> QDSTSDLIPAPPLSKVPLQQNFQDNQFQGKWYVVGLAGNAILREDKDPQKMYATIYELKEDKSYNVTSVLFRKKKCDYWIRTFVPGCQPGEFTLGNIKSYPGLTSYLVRVVSTNYNQHAMVFFKKVSQNREYFKITLYGRTKE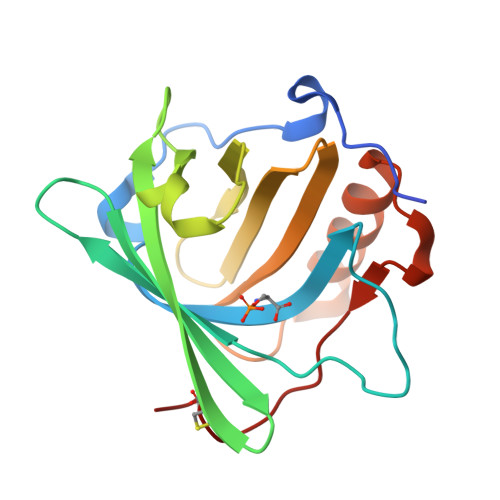LTSELKENFIRFSKSLGLPENHIVFPVPIDQCIDG> MELKLATAEKQVLDELVKLLQSRDLRGENGNWKEFLHVYDKNADSPSDPSRRSHEDLVQFLTTFKKKEDLQLLKCHANHLLIENLKQESQDEDTPEQMLVRLTVEHPSYSLDYSFKPYSEDWFVSDVGMKMKKVMESTNMVAVDCEMVLCEDGTEGLVRVGVVDRDLKVILDEFVKPNKPVVDYRTDITGITAEDIENASLSVVDIQETLQPFLSTGTILVGHSLNRDLEVLKIDHPKVIDTALVFKYPNTRKLRRPSLNNLCKSILGYEVRKTGVPHDCVHDASAAMKLALAVVEKRVDTTIKPSKEMLEVEKAKLFLHKIPNNVPSEELEQVLSGKFTLDVKQAKTQGRYYCAFALFHSS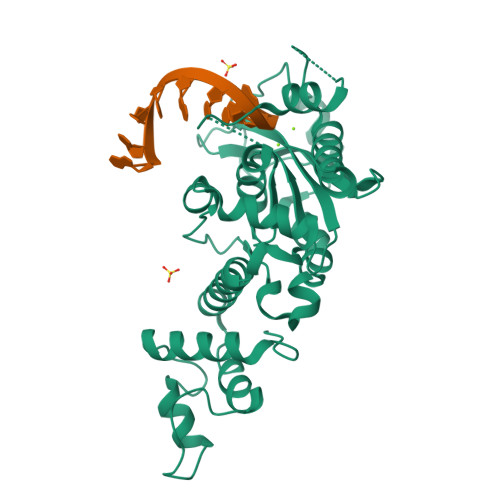EDADQAFEHIDGIEMTDSLGLPQKVVIIKLSSGSRASIYVRKMVQDE The human Casitas B lymphoma-b (Cbl-b) protein is a member of the monomeric Cbl family of RING-type E3 ubiquitin ligases that are known to downregulate non-receptor and receptor protein tyrosine kinase (PTK) signaling by ubiquitinating and thereby targeting these kinases for proteasomal or lysosomal degradation. The Cbl family of E3 ligases share a highly conserved N-terminal region that contains the structural elements required for ubiquitin ligase activity, including a substrate recognition tyrosine kinase-binding domain (TKBD), a short linker helix region (LHR) and a RING finger domain. The LHR comprises an N-terminal loop (linker loop 1), a helix, and a C-terminal loop (linker loop 2) and contains a strictly conserved tyrosine residue (Y363 in Cbl-b) within the linker helix (LH) that is essential for regulating the Cbl proteins E3 ligase activity. Specifically, Cbl-b is a negative regulator of signaling pathways involving immune cell receptors, and it is particularly well-documented to play a central role in inhibiting effector T cell activation.

To further characterize the C7683 interaction with Cbl-b and understand its mechanism of action, we co-crystallized the N-terminal E3 ligase fragment of Cbl-b containing the TKBD, LHR and RING domains (residue range 38–427) in complex with C7683. To improve the crystal packing and obtain better diffracting crystals, we introduced three-point mutations on the surface of the Cbl-b TKB domain by mutating residues K51, K55, R325 to alanines (the mutant protein referred to here as 3mCbl-b), which yielded crystals diffracting to 1.8 Å resolution. These mutations are located far from the substrate binding site as well as the regulatory regions involved in Cbl-b activation. A well-resolved electron density map was observed for the entire C7683 molecule and Cbl-b protein, except for residues 339–353 in the flexible linker helix region (LHR). C7683 was nestled in an interface between the 3 TKBD subdomains and the LHR, consistent with our biophysical studies, which showed that the compound binding does not involve the RING domain. C7683 binds in an extended conformation, making extensive interactions with the residues of all three TKBD subdomains, the LHR and coordinating a nearby water molecule (HOH10). The methyl-substituted piperidine ring is nestled in a pocket between the 4H and the SH2 subdomains, where it makes hydrophobic and van der Waals contacts with C289, T265, P71 and P72, in addition to a hydrogen bonding interaction between its nitrogen atom (N31) and the side chain oxygen (OE1) of E268 in the SH2 domain. The Isoindolin-1-one ring is also located between 4H and SH2 subdomains, making hydrophobic interactions with atoms from T144, K145, L148 in the 4H domain and L264 in the SH2, and hydrogen bonds to the backbone nitrogen of F263 in the SH2 domain through its oxygen atom.

> GQAAADRRTVEKTWALMDAVVRLCQNPKLQLKNSPPYILDILPDTYQHLRLILSKYDDNQKLAQLSENEYFKIYIDSLMKKSKRAIRLFKEGKERMYEEQSQDRRNLTKLSLIFSHMLAEIKAIFPNGQFQGDNFRITKADAAEFWRKFFGDKTIVPWKVFRQCLHEVHQISSGLEAMALKSTIDLTCNDYISVFEFDIFTRLFQPWGSILRNWNFLAVTHPGYMAFLTYDEVKARLQKYSTKPGSYIFRLSCTRLGQWAIGYVTGDGNILQTIPHNKPLFQALIDGSAEGFYLYPDGRSYNPDLTGLCEPTPHDHIKVTQEQFELYCEMGSTFQLCKICAENDKDVKIEPCGHLMCTSCLTAWQESDGQGCPFCRCEIKGTEPIIVDPFD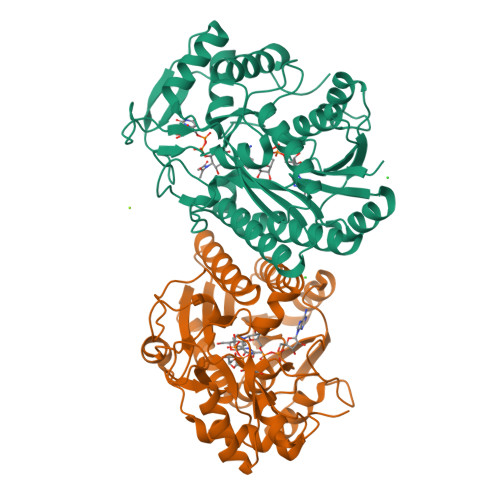>[2x]MAEKVLVTGGAGYIGSHTVLELLEAGYLPVVIDNFHNAFRGGGSLPESLRRVQELTGRSVEFEEMDILDQGALQRLFKKYSFMAVIHFAGLKAVGESVQKPLDYYRVNLTGTIQLLEIMKAHGVKNLVFSSSATVYGNPQYLPLDEAHPTGGCTNPYGKSKFFIEEMIRDLCQADKTWNVVLLRYFNPTGAHASGCIGEDPQGIPNNLMPYVSQVAIGRREALNVFGNDYDTEDGTGVRDYIHVVDLAKGHIAALRKLKEQCGCRIYNLGTGTGYSVLQMVQAMEKASGKKIPYKVVARREGDVAACYANPSLAQEELGWTAALGLDRMCEDLWRWQKQNPSGFGTQA The type III-E CRISPR-Cas system is a newly identified bifunctional complex with nuclease activity and protease activity that holds great potential for RNA editing applications. Here, we report cryo-electron microscopy (cryo-EM) structures of Desulfonema ishimotonii (Di) Cas7-11-crRNA, complexed with or without the full length or the N-terminus of TPR-CHAT. The Cas7 domains, arranged in a row, form a crescent-shaped filament, with the INS and CTE domain completing the structure. The Cas11 domain is positioned at the crescent’s midpoint, and interacts with Cas7.2 and Cas7.3.

For obtaining target RNA in the complex, we also obtained the structure using inactivated DiCas7-11-crRNA complex (DiCas7-11Inactive) by substituting the conserved catalytic residues, Cas7.2D429 and Cas7.3D654, with alanine to prevent cleavage of bound target RNA. However, the resulting complex did not reveal target RNA and exhibited no marked conformational changes to other structures.

> MTTTMKISIEFLEPFRMTKWQESTRRNKNNKEFVRGQAFARWHRNKKDNTKGRPYITGTLLRSAVIRSAENLLTLSDGKISEKTCCPGKFDTEDKDRLLQLRQRSTLRWTDKNPCPDNAETYCPFCELLGRSGNDGKKAEKKDWRFRIHFGNLSLPGKPDFDGPKAIGSQRVLNRVDFKSGKAHDFFKAYEVDHTRFPRFEGEITIDNKVSAEARKLLCDSLKFTDRLCGALCVIRFDEYTPAADSGKQTENVQAEPNANLAEKTAEQIISILDDNKKTEYTRLLADAIRSLRRSSKLVAGLPKDHDGKDDHYLWDIGKKKKDENSVTIRQILTTSADTKELKNAGKWREFCEKLGEALYLKSKDMSGGLKITRRILGDAEFHGKPDRLEKSRSVSIGSVLKETVVCGELVAKTPFFFGAIDEDAKQTALQVLLTPDNKYRLPRSAVRGILRRDLQTYFDSPCNAELGGRPCMCKTCRIMRGITVMDARSEYNAPPEIRHRTRINPFTGTVAEGALFNMEVAPEGIVFPFQLRYRGSEDGLPDALKTVLKWWAEGQAFMSGAASTGKGRFRMENAKYETLDLSDENQRNDYLKNWGWRDEKGLEELKKRLNSGLPEPGNYRDPKWHEINVSIEMASPFINGDPIRAAVDKRGTAVVTFVKYKAEGEEAKPVCAYKAESFRGVIRSAVARIHMEDGVPLTELTHSDCECLLCQIFGSEYEAGKIRFEDLVFESDPEPVTFDHVAIDRFTGGAADKKKFDDSPLPGSPARPLMLKGSFWIRRDVLEDEEYCKALGKALADVNNGLYPLGGKSAIGYGQVKSLGIKGDDKRISRLMNPAFDETDVAVPEKPKTDAEVRIEAEKVYYPHYFVEPHKKVEREEKPCGHQKFHEGRLTGKIRCKLITKTPLIVPDTSNDDFFRPADKEARKEKDEYHKSYAFFRLHKQIMIPGSELRGMVSSVYETVTNSCFRIFDETKRLSWRMDADHQNVLQDFLPGRVTADGKHIQKFSETARVPFYDKTQKHFDILDEQEIAGEKPVRMWVKRFIKRLSLVDPAKHPQKKQDNKWKRRKEGIATFIEQKNGSYYFNVVTNNGCTSFHLWHKPDNFDQEKLEGIQNGEKLDCWVRDSRYQKAFQEIPENDPDGWECKEGYLHVVGPSKVEFSDKKGDVINNFQGTLPSVPNDWKTIRTNDFKNRKRKNEPVFCCEDDKGNYYTMAKYCETFFFDLKENEEYEIPEKARIKYKELLRVYNNNPQAVPESVFQSRVARENVEKLKSGDLVYFKHNEKYVEDIVPVRISRTVDDRMIGKRMSADLRPCHGDWVEDGDLSALNAYPEKRLLLRHPKGLCPACRLFGTGSYKGRVRFGFASLENDPEWLIPGKNPGDPFHGGPVMLSLLERPRPTWSIPGSDNKFKVPGRKFYVHHHAWKTIKDGNHPTTGKAIEQSPNNRTVEALAGGNSFSFEIAFENLKEWELGLLIHSLQLEKGLAHKLGMAKSMGFGSVEIDVESVRLRKDWKQWRNGNSEIPNWLGKGFAKLKEWFRDELDFIENLKKLLWFPEGDQAPRVCYPMLRKKDDPNGNSGYEELKDGEFKKEDRQKKLTTPWTPWA> GGG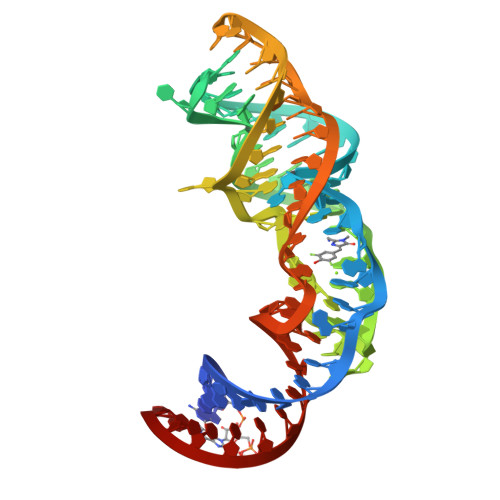AAGAUACAAGGUGAGCCCAAUAAUAUGGUUUGGGUUAGGAUAGGAAGUAGAGCCUUAAACUCUCUAAGCGGUAUCUUCCC>[2x]GLVAEAEAVAAGWMLDFLCLSLCRAFRDGRSEDFRRTRNSAEAIIHGLSSLTACQLRTIYICQFLTRIAAGKTLDAQ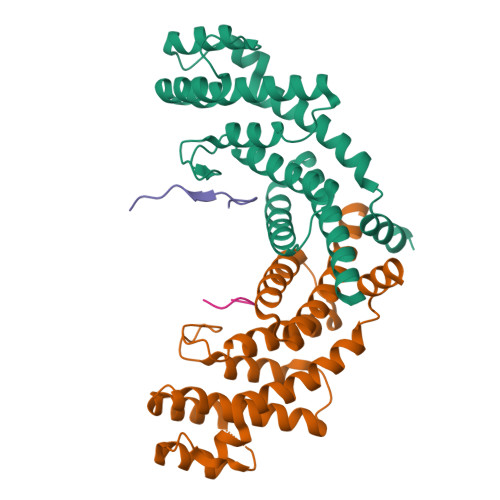FENDERITPLESALMIWGSIEKEHDKLHEEIQNLIKIQAIAVCMENGNFKEAEEVFERIFGDPNSHMPFKSKLLMIISQKDTFHSFFQHFSYNHMMEKIKSYVNYVLSEKSSTFLMKAAAKVVES;>KILLTPRRRQRL[2x]> MIDVIMTGELLKTVTRAIVALVSEARIHFLEKGLHSRAVDPANVAMVIVDIPKDSFEVYNIDEEKTIGVDMDRIFDISKSISTKDLVELIVEDESTLKVKFGSVEYKVALIDPSAIRKEPRIPELELPAKIVMDAGEFKKAIAAADKISDQVIFRSDKEGFRIEAKGDVDSIVFHMTETELIEFNGGEARSMFSVDYLKEFCKVAGSGDLLTIHLGTNYPVRLVFELVGGRAKVEYILAPRIES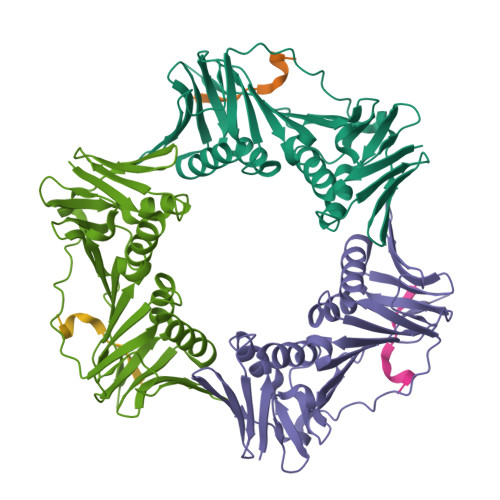E;> KSTQATLERWF N-[2-(1-FORMYL-2-METHYL-PROPYL)-1-(4-PIPERIDIN-1-YL-BUT-2-ENOYL)-PYRROLIDIN-3-YL]-METHANESULFONAMIDE 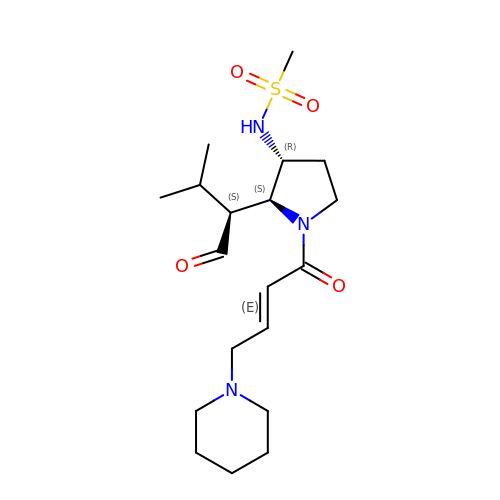| C19 H33 N3 O4 S | BSBJWRKWANAVRQ-POTLKAILSA-N N-(TRIS(HYDROXYMETHYL)METHYL)-3-AMINOPROPANESULFONIC ACID | C7 H17 N O6 S | 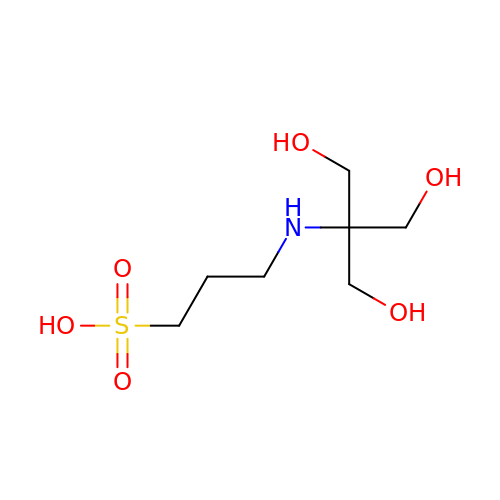YNLCVAQJIKOXER-UHFFFAOYSA-N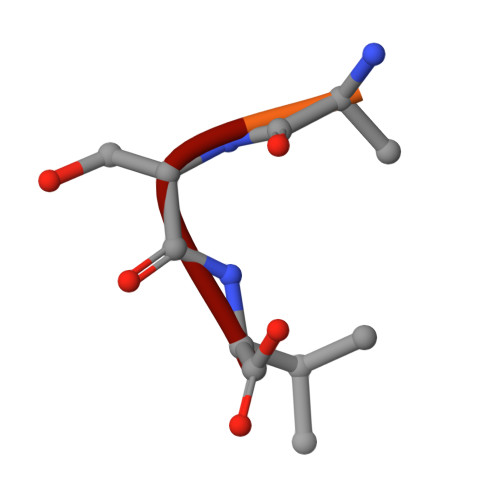> EVTSSV> GAMAPPRKVLIISAGASHSVALLSGDIVCSWGRGEDGQLGHGDAEDRPSPTQLSALDGHQIVSVTCGADHTVAYSQSGMEVYSWGWGNFGRLGHGNSSNLFTPLPIKALHGIRIKQIACGDSHCLAVTMEGEVQSWGRNQNGQLGLGDTEDSLVPQKIQAFEGIRIKMVAAGAEHTAAVTEDGDLYGWGWGRYGNLGLGDRTDRLVPERVTS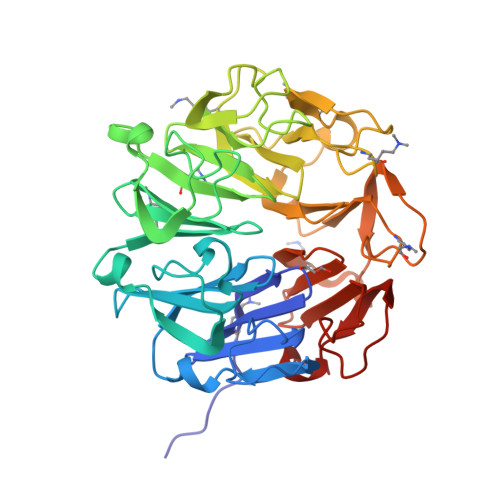TGGEKMSMVACGWRHTISVSYSGALYTYGWSKYGQLGHGDLEDHLIPHKLEALSNSFISQISGGWRHTMALTSDGKLYGWGWNKFGQVGVGNNLDQCSPVQVRFPDDQKVVQVSCGWRHTLAVTERNNVFAWGRGTNGQLGIGESVDRNFPKIIEALSVDG1-[3-({(2R)-2-[hydroxy(diphenyl)methyl]pyrrolidin-1-yl}sulfonyl)propyl]pyrimidine-2,4(1H,3H)-dione | C24 H27 N3 O5 S | 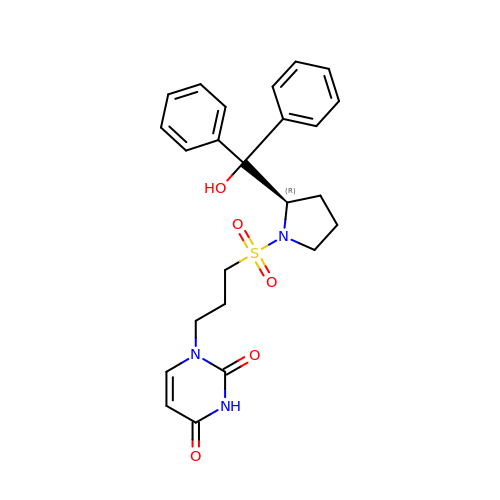NBGXNYZRJDHHHU-OAQYLSRUSA-N>[2x]GCCCGGAUGAUCCUCAGUGGUCUGGGGUGCAGGCUUCAAACCUGUAGCUG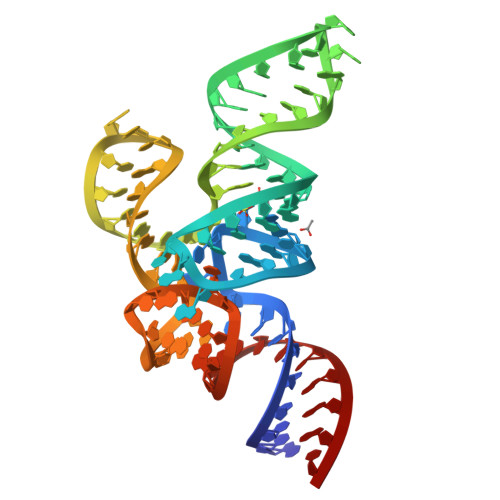UUUAGCGACAGAGUGGUUCAAUUCCACCUUUCGGGC>MASTKAPGPGEKHHSIDAQLRQLVPGKVSEDDKLIEYDALLVDRFLNILQDLHGPSLREFVQECYEVSADYEGKGDTTKLGELGAKLTGLAPADAILVASSILHMLNLANLAEEVQIAHRRRNSKLKKGGFADEGSATTESDIEETLKRLVSEVGKSPEEVFEALKNQTVDLVFTAHPTQSARRSLLQKNARIRNCLTQLNAKDITDDDKQELDEALQREIQAAFRTDEIRRAQPTPQDEMRYGMSYIHETVWKGVPKFLRRVDTALKNIGINERLPYNVSLIRFSSWMGGDRDGNPRVTPEVTRDVCLLARMMAANLYIDQIEELMFELSMWRCNDELRVRAEELHSSSGSKVTKYYIEFWKQIPPNEPYRVILGHVRDKLYNTRERARHLLASGVSEISAESSFTSIEEFLEPLELCYKSLCDCGDKAIADGSLLDLLRQVFTFGLSLVKLDIRQESERHTDVIDAITTHLGIGSYREWSEDKRQEWLLSELRGKRPLLPPDLPQTEEIADVIGAFHVLAELPPDSFGPYIISMATAPSDVLAVELLQRECGVRQPLPVVPLFERLADLQSAPASVERLFSVDWYMDRIKGKQQVMVGYSDSGKDAGRLSAAWQLYRAQEEMAQVAKRYGVKLTLFHGRGGTVGRGGGPTHLAILSQPPDTINGSIRVTVQGEVIEFCFGEEHLCFQTLQRFTAATLEHGMHPPVSPKPEWRKLMDEMAVVATEEYRSVVVKEARFVEYFRSATPETEYGRMNIGSRPAKRRPGGGITTLRAIPWIFSWTQTRFHLPVWLGVGAAFKFAIDKDVRNFQVLKEMYNEWPFFRVTLDLLEMVFAKGDPGIAGLYDELLVAEELKPFGKQLRDKYVETQQLLLQIAGHKDILEGDPFLKQGLVLRNPYITTL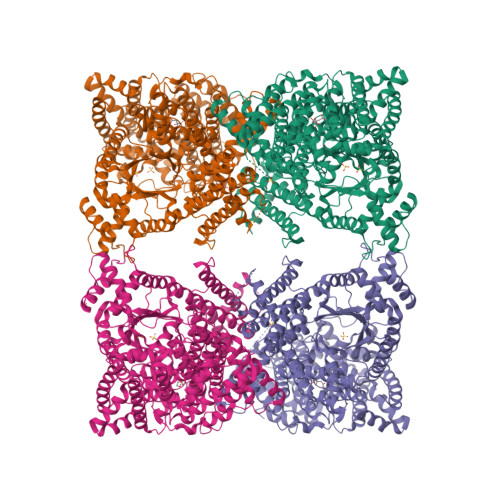NVFQAYTLKRIRDPNFKVTPQPPLSKEFADENKPAGLVKLNPASEYPPGLEDTLILTMKGIAAGMQNTG[8x]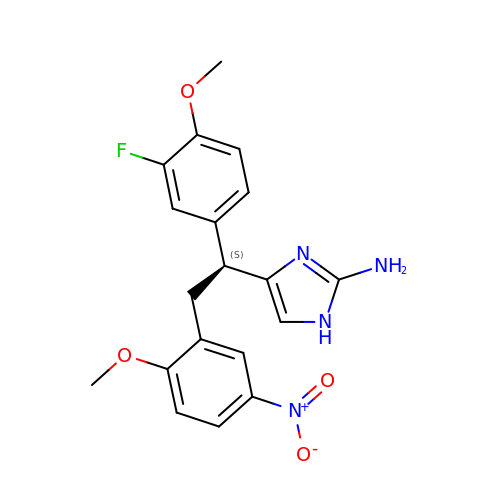4-[(1S)-1-(3-fluoro-4-methoxyphenyl)-2-(2-methoxy-5-nitrophenyl)ethyl]-1H-imidazol-2-amine | C19 H19 F N4 O4 | RFLOFHKRBGKCOB-AWEZNQCLSA-N> KQRGKEKV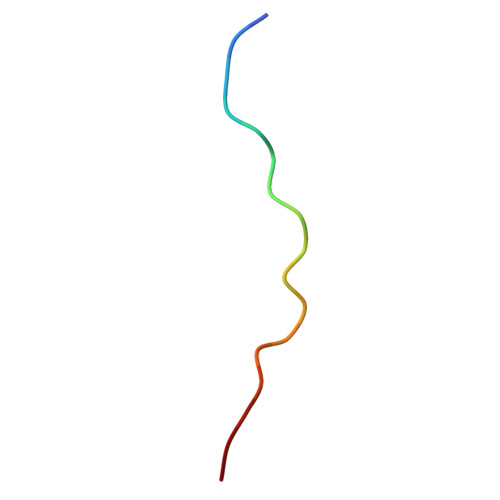SSGRPGQHN> RGGGDRGGFGPGK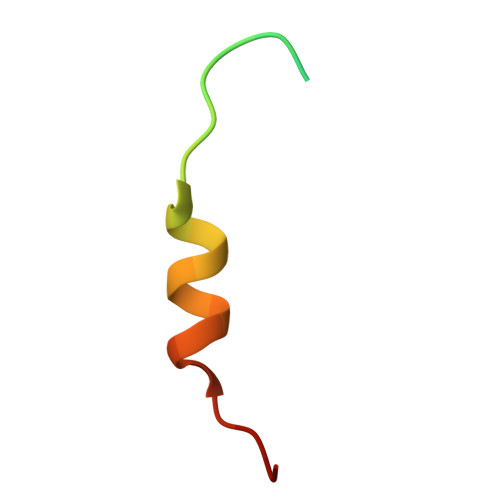MDSRGEHRQDRRERPY>MGSSHHHHHHSSGENLYFQGHMDVRIGQGYDVHQLVEGRPLIIGGVTIPYERGLLGHSDADVLLHAITDALFGAAALGDIGRHFSDTDAAFKGADSRVLLRACAERVKAAGFTIQNVDSTVIAQAPKLAPHIDGMRANIAADLGLPLERVNVKAKTNEKLGYLGRGEGIEAQAAALLVKQGG[3x]

2C-methyl-D-erythritol-2,4-cyclodiphosphate synthase (IspF) catalyzes the conversion of 4-diphosphocytidyl-2C-methyl-D-erythritol-2-phosphate to 2C-methyl-D-erythritol-2,4-cyclodiphosphate and cytidine monophosphate in production of isoprenoid-precursors via the methylerythritol phosphate biosynthetic pathway. IspF represents a potential target for development of broad-spectrum antimicrobial drugs since it is proven or inferred as essential in these pathogens and absent from mammals. In all IspF crystal structures three subunits form a compact bell-shaped assembly approximately 45 Å by 60 Å in the axial and equatorial dimensions respectively. The enzyme active site is located in a cleft at the interface of two subunits and here Zn2+ is coordinated by the side chains of two histidines and an aspartate.

Attempts to produce unliganded BcIspF crystals for ligand or fragment soaking experiments initially appeared to be successful and highly ordered samples were obtained. However, citrate was present in the best crystallization conditions and the electron density maps were consistent with this molecule coordinating the metal ion and therefore complicating ligand-binding studies. Citrate was well defined in one active site with an average B-factor of about 23 Å2, but less so in the other two where it was modeled with occupancy 0.75 and the average B-factors are approximately 37 and 43 Å2. For comparison, the average B-factor for protein atoms in this structure is approximately 19 Å2. The best-defined citrate binds to the active site Zn2+via both carboxylate and hydroxyl groups and this is also observed at one other site. Here the citrate forms hydrogen-bonding interactions with the main chain amides of His36 and Ser37, and side chains of Asp65 and Lys134. The interaction involving Asp65 is likely a consequence of the low pH at which crystals were obtained. The normally flexible and poorly ordered α2-α3 loop appears to lock down over the bound citrate adopting a configuration similar to that observed in the EcIspF-MEcPP complex. In the other citrate-binding pose (not shown) only a carboxylate coordinates to Zn2+ but hydrogen bonds are also formed exploiting the same functional groups on the protein, the amides of His36 and Ser37, Ser37 OG, and Lys134 NZ. It is clear from these results, that any attempts to investigate ligand binding at the Zn2+ site will require crystallization conditions that do not include citrate.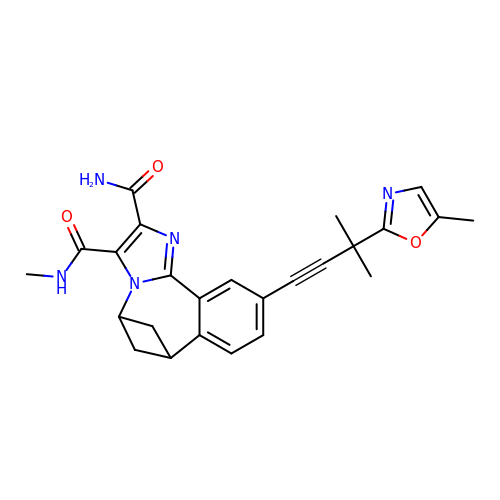(5s,7s)-N~3~-methyl-10-[3-methyl-3-(5-methyl-1,3-oxazol-2-yl)but-1-yn-1-yl]-6,7-dihydro-5H-5,7-methanoimidazo[2,1-a][2]benzazepine-2,3-dicarboxamide | C25 H25 N5 O3 | BVQAJAHFWBYNPF-IYBDPMFKSA-N> MAGQSDRKAALLDQV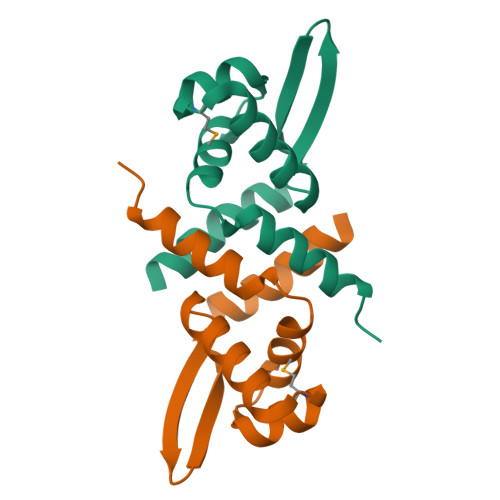ARVGKALANGRRLQILDLLAQGERAVEAIATATGMNLTTASANLQALKSGGLVEARREGTRQYYRIAGEDVARLFALVQVVADEHLEHHHHHH methyl (2Z)-3-[(3-chloro-1H-indol-7-yl)amino]-2-cyano-3-{[(3S)-2-oxo-1-(2-oxo-2-pyrrolidin-1-ylethyl)azepan-3-yl]amino}acrylate | C25 H29 Cl N6 O4 | 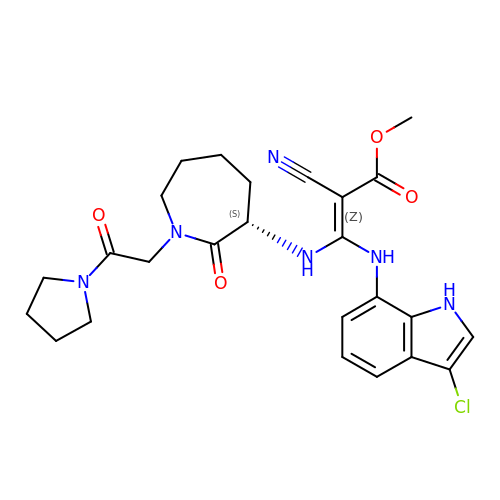QDGDCWKBZPDHTQ-UZXYXVAJSA-N Enterovirus 71 (EV71) is an emerging pathogen with pandemic potential. For human enteroviruses, binding of an entry receptor triggers a series of conformational changes, resulting in an “A-particle” that is primed for genome release. After endocytosis, an unknown trigger causes the A-particle to expel the viral genome, leaving behind an emptied capsid.

Purified EV71 mature virus was heated to 56°C for 12 minutes to produce A-particles. To elucidate the structural rearrangements that occur during the EV71 uncoating process, we have reconstructed high-resolution cryo-electron microscopy (cryoEM) maps of the A-particle (6.3 Å) and empty capsid (9.2 Å). The A-particle interior contained density corresponding to the RNA genome, whereas the empty capsid was completely devoid of internal density. The A-particle two-fold openings are larger in diameter and the internal capsid residues link the protein shell to the viral RNA. The two-fold opening in the A-particle has a measured diameter of 9.3 Å, whereas the empty capsid has an opening of only 6.4 Å, a 2.9 Å difference. This size difference suggests that the diameter of the channel is linked to the presence or absence of RNA. Over all, these two-fold channels are broader and more open in the A-particle, likely to facilitate the release of ordered RNA, an important feature as the termini of the picornavirus genome retains large amounts of secondary structure. The A-particle shows that the interior surface has large patches of negative charge at the two-fold axis of symmetry with minimal interspersed positive charges. In contrast, the five-fold vertex is lined with positively and neutrally charged residues. When the capsid interacts with its receptor on a host cell membrane the pocket factor is expelled from the base of the canyon. This release allows the capsid to expand and open the two-fold channels, leading to formation of the A-particle, in which a portion of the N-terminus of VP1 is tethered to the RNA genome.

> HSTAETTLDSFFSRAGLVGEIDLPLKGTTNPNGYANWDIDITGYAQMRRKVELFTYMRFDAEFTFVACTPTGEVVPQLLQYMFVPPGAPKPDSRESLAWQTATNPSVFVKLSDPPAQVSVPFMSPASAYQWFYDGYPTFGEHKQEKDLEYGAMPNNMMGTFSVRTVGTSKSKYPLVVRIYMRMKHVRAWIPRPMRNQNYLFKANPNYAGNSIKPTGASRTAITTL;> VAQLTIGNSTITTQEAANIIVGYGEWPSYCSDSDATAVDKPTRPDVSVNRFYTLDTKLWEKSSKGWYWKFPDVLTETGVFGQNAQFHYLYRSGFCIHVQCNASKFHQGALLVAVLPEYVIGTVAGGTGTEDTHPPYKQTQPGADGFELQHPYVLDAGIPISQLTVCPHQWINLRTNNCATIIVPYINALPFDSALNHCNFGLLVVPISPLDYDQGATPVIPITITLAPMCSEFAGLR;> GFPTELKPGTNQFLTTDDGVSAPILPNFHPTPCIHIPGEVRNLLELCQVETILEVNNVPTNATSLMERLRFPVSAQAGKGELCAVFRADPGRNGPWQSTLLGQLCGYYTQWSGSLEVTFMFTGSFMATGKMLIAYTPPGGPLPKDRATAMLGTHVIWDFGLQSSVTLVIPWISNTHYRAHARDGVFDYYTTGLVSIWYQTNYVVPIGAPNTAYIIALAAAQKNFTMKLCKDASDILQTG N-[2,6-di(propan-2-yl)phenyl]-N'-(N-ethylcarbamimidoyl)urea | C16 H26 N4 O | 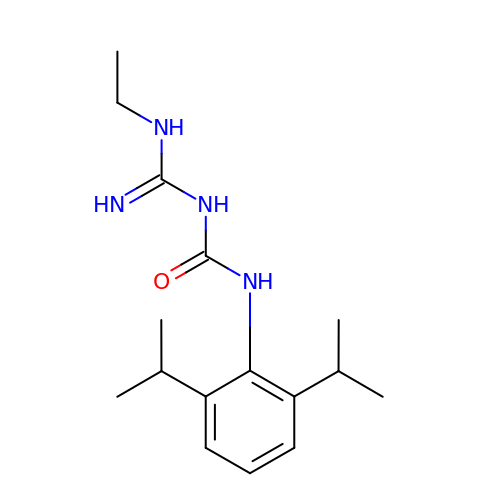ABOWUZLWUNTBAJ-UHFFFAOYSA-N>MALVDGFLELERSSGKLEWSAILQKMASDLGFSKILFGLLPKDSQDYENA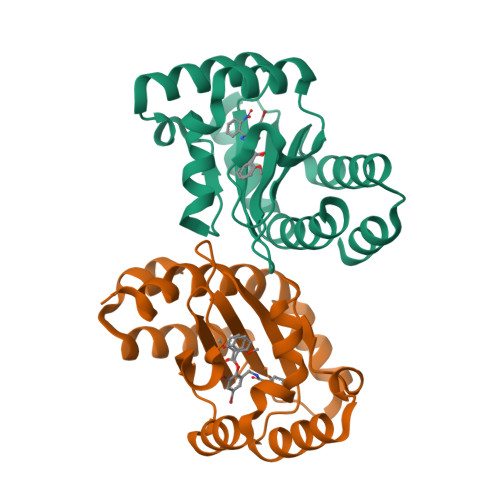FIVGNYPAAWREHYDRAGYARVDPTVSHCTQSVLPIFWEPSIYQTRKQHEFFEEASAAGLVYGLTMPLHGARGELGALSLSVEAENRAEANRFMESVLPTLWMLKDYALQSGAGLAFEHP[12x]> MNTKYNKEFLLYLAGFVDGDGSIIAQIKPNQSSKFKHRLSLTFQVTQKTQRRWFLDKLVDEIGVGYVRDSGSVSNYILSEIKPLHNFLTQLQPFLKLKQKQANLVLKIIEQLPSAKESPDKFLEVCTWVDQIAALNDSKTRKTTSETVRAVLD;> MNTKYNKEFLLYLAGFVDGDGSIIAQIE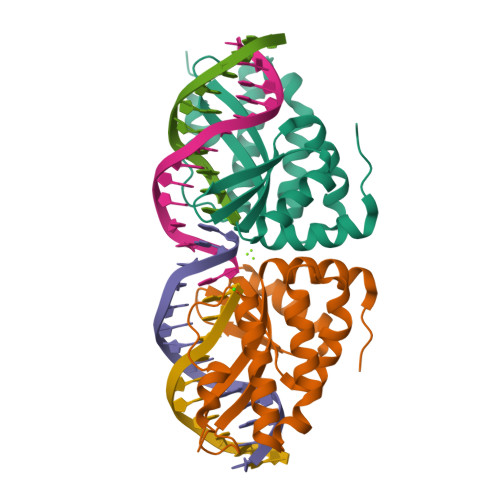PNQSYKFKHRLKLTFKVTQKTQRRWFLDKLVDEIGVGYVSDSGSVSNYILSEIKPLHNFLTQLQPFLKLKQKQANLVLKIIEQLPSAKESPDKFLEVCTWVDQIAALNDSKTRKTTSETVRAVLD The human SMC5/6 complex is a conserved guardian of genome stability and an emerging component of antiviral responses. Here, we identify a novel SMC5/6 subunit called SIMC1 that contains SUMO interacting motifs (SIMs) and an Nse5-like domain. SIMC1’s Nse5-like domain binds to the putative Nse6 orthologue SLF2 to form an anti-parallel helical dimer resembling the yeast Nse5/6 structure. Thus, two Nse5/6-like complexes with distinct recruitment domains control human SMC5/6 localization.

To evaluate the accuracy of the predicted structures, we performed cryo-EM single-particle analysis on the SIMC1284-SLF2CTD complex. 3D reconstruction yielded an anisotropic and low-quality map, resolving side-chain densities of only bulky residues in the protein core. Nonetheless, the predicted SIMC1-SLF2 model could be docked into the map unambiguously and refined to ~3.9 Å resolution. The refined structure was strikingly similar to the predictions, with r.m.s.d.s of only ~1 Å for Cα atoms, validating the accuracy of the predicted structures. The cryo-EM structure contains 425–858 aa of SIMC1 and 733–1158 aa of SLF2. SIMC1 and SLF2 α-solenoids face each other in a head-to-tail fashion through the concave surfaces of their slightly curved shapes. Overall, the ellipsoid-shaped SIMC1-SLF2 structure resembles the Nse5/6 structure. A notable feature of the SIMC1-SLF2 structure is that the most N-terminal region (425–467 aa) of SIMC1 preceding its α-solenoid adopts an extended conformation, and a short region (431–451 aa) within it adopts a loop-like conformation that inserts into a cleft between the curved SIMC1 and SLF2 α-solenoids. The loop contributes directly to the formation of the SIMC1-SLF2 interface; without this loop, the α-solenoids’ interface would bury a surface area of only ~1500 Å2, but the complete interface including the loop buries ~2500 Å2. The interaction surfaces of both SIMC1 and SLF2 are highly charged.

> AYLQDMPRSPGDVPQSPSDVSPSPDAPQSPGGMPHLPGDVLHSPGDMPHSSGDVTHSPRDIPHLPGDRPDFTQNDVQNRDMPMDISALSSPSCSPRPQSETPLEKVPWLSVMETPARKEISLSEPAKPGSAHVQSRTPQGGLYNRPCLHRLKYFLRPPVHHLFFQTLIPDKDTRENKGQRLEPIPHRRLRMVTNTIEENFPLGTVQFLMDFVSPQHYPPREIVAHIIQKILLSGSETVDVLKEAYMLLMKIQQLHPANAKTVEWDWKLLTYVMEEEGQTLPGRVLFLRYVVQTLEDDFQQTLRRQRQHLQQSIANMVLSCDKQPHNVRDVIKWLVKAVTEDGLTQPPNGNQTSSGTGILKASSSHPSSQPNLTKNTNQLIVCQLQRMLSIAVEVDRTPTCSSNKIAEMMFGFVLDIPERSQREMFFTTMESHLLRCKVLEIIFLHSCETPTRLPLSLAQALYFLNNSTSLLKCQSDKSQWQTWDELVERLQFLLSSYQHVLREHLRSSVIDRKDLIIKRIKPKPQQGDDITVVDVEKQIEAFRSRLIQMLGEPLVPQLQDKVHLLKLLLFYAADLNPDAEPFQKGWSGS;> TPAATGKPPALSKGLRSQSSDYTGHVHPGTYTNTLERLVKEMEDTQRLDELQKQLQEDIRQGRGIKSPIRIGEEDSTDDEDGLLEEHKEFLKKFSVTIDAIPDHHPGEEIFNFLNSGKIFNQYTLDLRDSGFIGQSAVEKLILKSGKTDQIFLTTQGFLTSAYHYVQCPVPVLKWLFRMMSVHTDCIVSVQILSTLMEITIRNDTFSDSPVWPWIPSLSDVAAVFFNMGIDFRSLFPLENLQPDFNEDYLVSETQTTSRGKESEDSSYKPIFSTLPETNILNVVKFLGLCTSIHPEGYQDREIMLLILMLFKMSLEKQLKQIPLVDFQSLLINLMKNIRDWNTKVPELCLGINELSSHPHNLLWLVQLVPNWTSRGRQLRQCLSLVIISKLLDEKHEDVPNASNLQVSVLHRYLVQMKPSDLLKKMVLKKKAEQPDGIIDDSLHLELEKQAYYLTYILLHLVGEVSCSHSFSSGQRKHFVLLCGALEKHVKCDIREDARLFYRTKVKDLVARIHGKWQEIIQNCRPTQGQLHDFWVPDS>MKRHHHHHHGSGDLVAWNKENDRRTLWTTPDPEANCKVSEEKDSKLTLVLTKCGSQILASVSLLVVKGKFANINNKTNPGEDYKKFSVKLLFDANGKLLTGSSLDGNYWNYKNKDSVIGSPYENAVPFMPNSTAYPKIINNGTANPEDKKSAAKKTIVTNVYLGGDAAKPVAT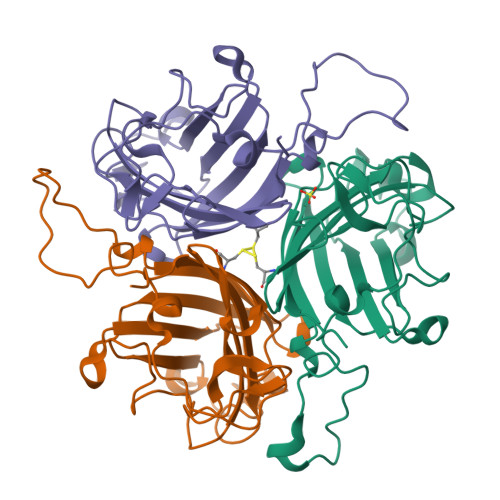TISFNKETESNCVYSITFDFAWNKTYKNVPFDSSSLTFSYIAQDAEDKNE[6x]> AAVVASLKPLGFIASAIADGVTDTQVLLPDGASEHDYSLRPSDVKRLQGADLVVWVGPEMEAFMEKSVRNIPDNKQVTIAQLADVKPLLMKGADDDEDEHAHTGADEEKGDVHHHHGEYNMHLWLSPEIARATAVAIHEKLVELMPQSRAKLDANLKDFEAQLAATDKQVGNELAPLKGKGYFVFHDAYGY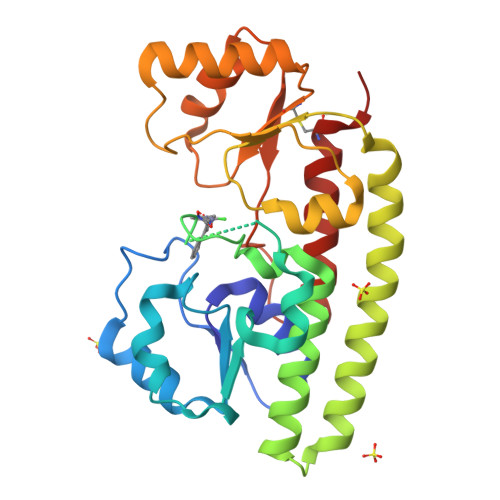YEKHYGLTPLGHFTVNPEIQPGAQRLHEIRTQLVEQKATCVFAEPQFRPAVVEAVARGTSVRMGTLDPLGTNIKLGKTSYSAFLSQLANQYASCLKGD>MEQRASLDSEESESPPQENSCLDPPDRDPNCKPPPVKPHIFTTRSRTRLFGKGDSEEASPLDCPYEEGGLASCPIITVSSVLTIQRPGDGPASVRPSSQDSVSAGEKPPRLYDRRSIFDAVAQSNCQELESLLPFLQRSKKRLTDSEFKDPETGKTCLLKAMLNLHNGQNDTIALLLDVARKTDSLKQFVNASYTDSYYKGQTALHIAIERRNMTLVTLLVENGADVQAAANGDFFKKTKGRPGFYFGELPLSLAACTNQLAIVKFLLQNSWQPADISARDSVGNTVLHALVEVADNTVDNTKFVTSMYNEILILGAKLHPTLKLEEITNRKGLTPLALAASSGKIGVLAYILQREIHEPECRHLSRKFTEWAYGPVHSSLYDLSCIDTCEKNSVLEVIAYSSSETPNRHDMLLVEPLNRLLQDKWDRFVKRIFYFNFFVYCLYMIIFTAAAYYRPVEGLPPYKLKNTVGDYFRVTGEILSVSGGVYFFFRGIQYFLQRRPSLKSLFVDSYSEILFFVQSLFMLVSVVLYFSQRKEYVASMVFSLAMGWTNMLYYTRGFQQMGIYAVMIEKMILRDLCRFMFVYLVFLFGFSTAVVTLIEDGKNNSLPMESTPHKCRGSACKPGNSYNSLYSTCLELFKFTIGMGDLEFTENYDFKAVFIILLLAYVILTYILLLNMLIALMGETVNKIAQESKNIWKLQRAITILDTEKSFLKCMRKAFRSGKLLQVGFTPDGKDDYRWCFRVDEVNWTTWNTNVGIINEDPGNCEGVKRTLSFSLRSGRVSGRNWKNFALVPLLRDASTRDRHATQQEEVQLKHYTGSLKPEDAEVFKDSMVPGEK[4x]

Here we present a model refinement protocol that automatically generates series of molecular models from CryoEM datasets, which describe the dynamics of the macromolecular system and have near-perfect geometry scores. Here, we present a computational method, similarly based on the GMM-DNN architecture, that builds a series of molecular models from a CryoEM dataset with structural variability. Each model in the ensemble would satisfy protein geometry constraints and fit to the reconstruction of particles from the same conformation at the target resolution. In addition to the FSC, we also introduce stereochemical constraints of proteins and RNAs to the loss function during DNN training, which ensures that the model at every frame along the trajectory has valid geometry.

To demonstrate the protocol, we start with a classical modeling task, where one atomic model is refined against one high-resolution CryoEM structure. The process involves large-scale morphing, residue-wise adjustment, and finally full atom refinement that considers both the map-model agreement and the stereochemical constraints. The modeling process starts from an existing homolog or predicted model, where we place one Gaussian function at each non-hydrogen atom. Using a DNN, we first refine the GMM so it fits the consensus 3D reconstruction of all particles. During the refinement, the map-model Fourier shell correlation (FSC) is used to guide the model fitting, and a cutoff frequency is set to avoid over-interpreting the high-resolution information in the map. In sum, for single model refinement tasks, our atomic model refinement protocol produces better models than results from existing methods, according to the PDB validation metrics. We again start from the TRPV1 example (EMPIAR-10059), from which the movement of Ankyrin repeat domains has been observed previously.>MEHRAFKWPQPLAGNKPRIWYGGDYNPDQWPEEVWDEDVALMQQAGVNLVSVAIFSWAKLEPEEGVYDFDWLDRVIDKLGKAGIAVDLASGTASPPMWMTQAHPEILWVDYRGDVCQPGARQHWRATSPVFLDYALNLCRKMAEHYKDNPYVVSWHVSNAYGCHNRFDYSEDAERAFQKWCEKKYGTIDAVNDAWGTAFWAQRMNNFSEIIPPRFIGDGNFMNPGKLLDWKRFSSDALLDFYKAERDALLEIAPKPQTTNFMVSAGCTVLDYDKWGHDVDFVSNDHYFSPGEAHFDEMAYAACLTDGIARKNPWFLMAHSTSAVNWRPTNYRLEPGELVRDSLAHLAMGADAICYFQWRQSKAGAEKWHSAMVPHAGPDSQIFRDVCELGADLNKLADEGLLSTKLVKSKVAIVFDYESQWATEHTATPTQEVRHWTEPLDWFRALADNGLTADVVPVRGPWDEYEAVVLPSLAILSEQTTRRVREYVANGGKLFVTYYTGLVDDRDHVWLGGYPGSIRDVVGVRVEEFAPMGTDAPGTMDHLDLDNGTVAHDFADVITSVADTAHVVASFKADKWTGFDGAPAITVNDFGDGKAAYVGARLGREGLAKSLPALLEELGIETSAEDDRGEVLRVERADETGENHFVFLFNRTHDVAVVDVEGEPLVASLAQVNESEHTAAIQPNGVLVVKLAAALEHHHHHH[6x]

Aim: Bifidobacterium longum subsp. infantis uses a glycoside hydrolase (GH) family 42 β-galactosidase (BiBga42A) for hydrolyzing lacto-N-tetraose (LNT), which is the most abundant core structure of human milk oligosaccharides (HMOs). As such, BiBga42A represents one of the pivotal enzymes underpinning the symbiosis between bifidobacteria and breastfed infants. BiBga42A has a three-dimensional structure similar to other GH42 enzymes that have three domains consisting of a (β/α)8 barrel (domain A), an α/β fold (domain B), and an anti-parallel β-sandwich (domain C). Glu-160 and Glu-318 in BiBga42A were predicted to be the acid/base catalyst and the nucleophile, respectively, based on previous studies of GH42 enzymes and sequence alignment.

Therefore, we also replaced the acid/base catalyst Glu-160 with alanine and performed co-crystallization with LNT using the preparation (E160A/E318A double mutant). However, LNT was also hydrolyzed during the crystallization under these conditions, because only the electron density of the product Gal in the α-configuration (α-Gal) was observed in subsite -1 of the active site. The Gal-complexed structure was determined at 1.9 Å resolution (E160A/E318A-Gal). α-Gal was also observed in the crystal structures of several other GH42 enzymes[23-26]. The asymmetric unit contained six molecules (two trimers) of BiBga42A. The main chain structures of the six polypeptides (chains A-F) were virtually the same (Cα RMSD < 0.107 Å for all chain pairs), and an α-Gal molecule was similarly bound in each chain. The pyranose ring of the α-Gal adopts an undistorted 4C1 conformation, and the C6 hydroxyethyl group takes a gt conformation. The O6 atom of the sugar forms hydrogen bonds with the side chain nitrogen atoms of Trp-326 and His-369, while the axial O4 atom is recognized by Arg-121 and Glu-366. The O2 atom of the Gal makes hydrogen bonds with the side chains of Asn-159 and Asp-285. The α-anomeric O1 atom is recognized by the side chains of Asp-285 and Tyr-287 via hydrogen bonds. The side chain of Phe-356 makes a stacking interaction with the hydrophobic C4 region of the pyranose ring.4-(4-METHYL-PIPERAZIN-1-YLMETHYL)-N-[4-METHYL-3-(4-PYRIDIN-3-YL-PYRIMIDIN-2-YLAMINO)-PHENYL]-BENZAMIDE | C29 H31 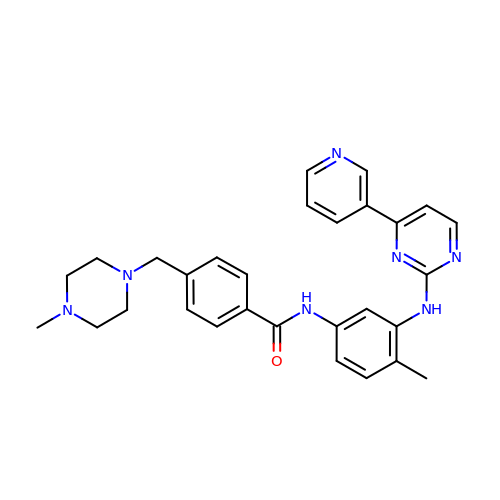N7 O | KTUFNOKKBVMGRW-UHFFFAOYSA-N>[3x]GSHMFKVKKLSDKAIIPQRGSKGAAGYDLSSAHELVVPAHGKALAMTDLQIAIPDGTYGRIAPRSGLAWKNFIDCGAGVIDSDYRGNVGVVLFNHSDVDFKVAVGDRVAQLIFERIVTPEPLEVDEIDETQRGAGGFGSTGVKVQN

To understand how the pyrimidine biosynthesis pathway accommodates the demand for dTTP, we began to focus on a key enzyme of the pathway, deoxyuridine triphosphate nucleotidohydrolase or dUTPase, which hydrolyzes dUTP to pyrophosphate and dUMP; dUMP is subsequently converted to dTTP. Concomitantly, a high dTTP to dUTP ratio is ensured, thus minimizing the incorporation of uracil during DNA synthesis. The curated genome of the soil amoeba D. discoideum shows a single gene (DictyBase Gene ID DDB_G0293374;) predicted to encode a dUTPase polypeptide containing the five hallmark motifs (M1–M5) of homotrimeric dUTPases, seen in the alignments of the amino acid sequences from mustard, yeast and human. While the dUTPases of Arabidopsis thaliana and D. discoideum have substantial stretches of identity (73%) within the 138-residue segment containing M1–M5, their N-termini have very low sequence similarity to each other, and to the human and yeast N-termini. Notably, within the lengthy N-terminus of the D. discoideum dUTPase, atypical of most dUTPases, computational analyses predict a mitochondrial targeting sequence (MTS).

Also catalytically-active was a core version comprised of polypeptide subunits that retain M1–M5 but lack residues 1-37 of the N-terminus. A homotrimeric structure of the core dUTPase enzyme was confirmed by crystallographic analyses that additionally showed interactions of the shorter N-termini with the C-termini likely enhanced substrate access of the dUTP substrate to the active sites. In most homotrimeric dUTPases, the C-termini, containing M5 which aids in coordinating the ligand at the active site, are flexible. In the core structure, PISA interaction analyses revealed that the shorter N-termini interacted with the C-termini of adjacent subunits, constraining their engagement with their respective active sites. The limited movement of the C-termini contributed to the different inhibitor coordinates in each active site of the core dUTPase (insets). Notable is the position of Inhibitor B. Interactions (hydrogen bonds and salt bridges) by three glutamates of the C-terminus of Chain C with residues of the N-terminus of Chain A (E120::H3+F5, E123::K5 and E126::K9) produced the most displaced orientation compared to Inhibitors A and C (detailed in Additional file 3: Fig. S3). The C-termini, which act normally as lids for the substrate binding pockets, instead were restricted in their movement, which may have allowed increased access of dUTP to the three active sites compared to the full-length protein with its extended N-termini.> MEFINSFNLVMSNIFDNHNNSSIEFWRICEQINYFQNLWFRIHDDLIISSFKLMGSLARCNTNEVFNFFAQGSAQFTWAKLFQNFSSYAHALNSIEFSQSIQSNQMNSSTTTTQQISSTPQQHQQHQQQQQQQQGYNNQQIPNTPYQQFQPTMQYQGQQSSMQQSVGQQQQPQQQPQQQNTPNTPNSTTSSNTANTTSPVKITQLLLSEKDSDALSSIFQLISRLVESSMAVGNVFLKIGPLISLAFQFAVSQVDSKLKSSALSVITSYSQYPIYVADIWRLINETNLFNSGLSAIGGLNELSFTQQSLELLLQLIQQSSFLFDKSNHYQESLKLKSYLDSCMDLFNLLNIKSFNTLDEKWKFALTLMKIFEFSIIQFNQSIQNFQIDKQHPCYQLYIELNRSSLSSNLYQQQQQQQNKYQQQQQQQQQSKKTTLENIIKIIDYSNDQSILIQQQIQQQQQQQQQGYNQDSSRVILNLVFQQLQQQDNDDFNLLVLKCLDLLLLISDNTVYDIENAKSLVVNLSNMDYSRPIVSIAKLIDHELPAISLRAIRLIYSFECYTHQISTVFLDSDPNLILSKFIKMMEFNESNFEDFSGTNYDQTISFIRYASNSVQWTIAQLIMLCLSNISSGRYTLAHFLLGCSSNLDLSKDFIPNSKSCLTLIIKNVMNSQFVERYPHLVDCYHEIIWKMSSDPITWKPMIKYIQEEFPNYYHDSLLILRNAITINGSSERRTEALISSMSWVFKTCSISIQNSYSIEMKQFLTRLIFPSLMNLNQPSMNGGIGGLNGTINNGLIMGISPINILSLYNTIEFQLPEINRPRIFSMYPNLIEYFTTNININNLNSNNNNNNNNNNNNNNNNNNNNNNNNNNNNNNNNNNNNNNNNITNGGTSQLLDIIKIREVLKNDFNRFSNEFEIERELEECCLINSSIQLYNSKLKALDGWKSFINISLAQNTIEIDTLDESLLLSLLQRIVIDFSNERNPIESTLSIGYTILTILFTLKLKKDSYQLFINSSLTTNSTDSNVIEQKMKSIFEGLLQTVLKSPHQAIRGISYTCLIQYLDLSATTPTTPSLSPLSTSINNVVEMNNK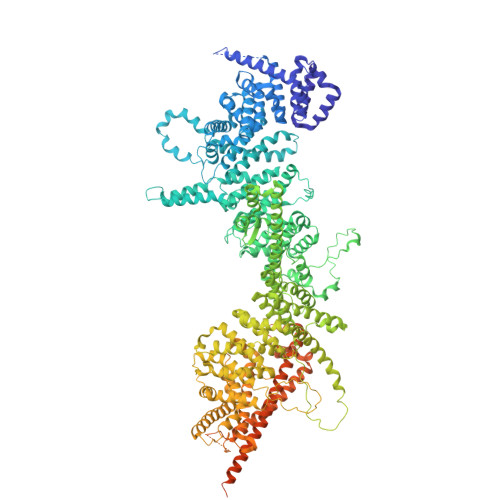SKNKNNQDKEQGYGNLNIGLIISKIEDKFIRILSSDCNSFSRGWRITAISCMQSILSIDNLCGHRSLMFLQNKGFIINMINDTCSKYLSDNWENIDPKDLHVYKSQMSLLLKISQQMDGVHLLMNNNVIGSFVKSPFLNYIPTDKIFGKFIEILLPILQLFASLCCYCNNTSKNNGNINNNNNVGGTVLIGSDRNEIYQELFDFLSNHSDLFIIILSDQSSFSHPTLSSLKVLKLTCFLFSKVSSLFFKKSTTTSSSTSTTSSHNRTQFNRFHYCLINLLVKYSVNSKQIIELVKPENIDEELLTEKIDFSYLPKSSIENQFKNIPDDINIGGVNIGLTSKNSNNNNNNNNNNNGSINGKKSKRKNQFQILIKETITSIIHDLLLYCRKVSIVQDSNFGFVCFNSNLNIYQQFQSFSSLRSTNRNNSNNNNINNNNNNNSNNNYNNNSMNSDMDNDDDNIINNNSYKFNNKNNNNNNDNNNQNKNSIFGGFGVNNSIINGNNNNNNGNNNNNNGNNGVNILPSIDLAINILVDNILQYSFYKVDLSQCFKLLQSYDQLTNYQYQEILQTGEDYPAFGPTQRNHMVENILKEKIIDIETQISIIHENIEILLLLIVSHSFYFCNSLYLLFQNSNNNFYSSAIGGTISPTLASSAYYPTTQQQQQQQQQGGSNLKITDLNASTTTSNIKKNNESAFLSSKTNQNSGGMLSSVFSYFKGQQNNTPSAQVSQIPINSTPYSTNYATPHQHQQLLQQQQQRQQQIQQQINQTPSNELSPQEIEVFLKRLKQSIFEREVNQLGGKLSDVILNQIDKKSTLIDLLLKKLQDLTK> 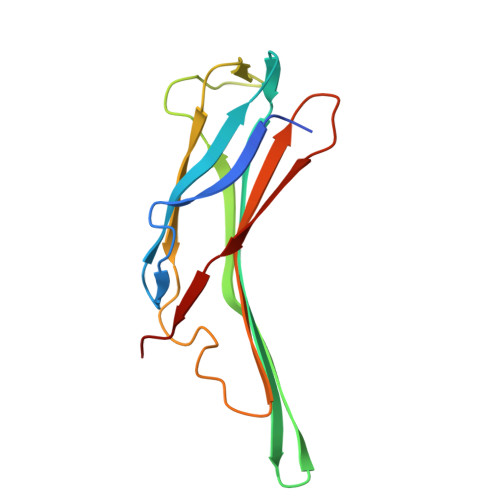SNVMFKKIKSFEVVFNDPEKVYGSGERVAGRVIVEVSEVTRVKAVRILASGVAKVLWMQGSQQCAQTSEYLRYEDTLLLEDQPTGENEMVIMRPGNKYEYKFGFELPQGPLGTSFKGKYGSVDYWVKAFLDRPSQPTQETKKNFEVVDLV>[2x]EWQENKSWNAHFTEHKSQGVVVLWNENKQQGFTNNLKRANQAFLPASTFKIPNSLIALDLGVVKDEHQVFKWDGQTRDIATWNRDHNLITAMKYSVVPVYQEFARQIGEARMSKMLHAFDYGNEDISGNVDSFWLDGGIRISATEQISFLRKLYHNKLHVSERSQRIVKQAMLTEANGDYIIRAKTGYSTRIEPKIGWWVGWVELDDNVWFFAMNMDMPTSDGLGLRQAITKEVLKQEKIIP

Prevalently, drug-resistant bacteria produce β-lactamase enzymes that hydrolyze and inactivate the β-lactam ring, thus preventing the covalent inhibition of essential cell-wall biosynthesis proteins, named penicillin-binding proteins (PBPs), which result in the loss of drug’s antibacterial effectiveness. OXA-48 belongs to the carbapenem-hydrolyzing class D β-lactamases (CHDLs) and together with its variants represents one of the most severe threat of resistance, compromising efficacious anti-infective treatments. Isolated for the first time in 2001 from a patient in Turkey, the OXA-48 enzyme is now widespread across the world and is commonly identified in Escherichia coli and Klebsiella pneumoniae. We then prioritized the 4-ideneamino-4H-1,2,4-triazole (SC_2) and pyrazolo[3,4-b]pyridine (SC_7) derivatives for further investigation and demonstrated by biochemical and X-ray studies a reversible and competitive binding mode within OXA-48 active site for both series.

Importantly, the most potent representative of the latter series (ID2, AC50 = 0.99 μM) inhibited OXA-48 via a reversible and competitive mechanism of action, as demonstrated by biochemical and X-ray studies; furthermore, it slightly improved imipenem’s activity in Escherichia coli ATCC BAA-2523 β-lactam resistant strain. The overall density was unambiguous and both chains included the carboxylated form of Lys73 residue. A salt bridge and hydrogen bonds between the positively charged Arg250 and the benzoic acid moiety were observed. The carboxylate group was also oriented in such a way that also Lys208 participated in an ionic bond. Additionally, the distances between the carboxylic oxygen and the hydroxyl group of Thr209 and Ser118 below 3.0 Å were consistent with the formation of hydrogen bonds. Moving on the upper part of the binding pocket, Arg214 established a salt bridge and hydrogen bonds with the 4-COOH group, as well as a cation–π interaction with the phenylethyl moiety of the ligand. The carboxylate group on the pyrazolo[3,4-b]pyridine core was also involved in a water bridge hydrogen bond with Thr213 and Tyr211. Moreover, the central bicyclic aromatic system of the ligand established a π–π interaction with Trp105. Overall, an unambiguous binding mode was obtained consistent with that seen for reversible compound ID3, where dianionic moieties clearly engage the positively charged Arg214 and Arg250. The obtained crystal structure therefore proved compound ID2 to occupy OXA-48 binding pocket with a reversible MoA in line with the aforementioned experimental results.>MSLSAKSSLKEVAELAGVGYATASRALSGKGYVSPQTREKVQAAAKELNYVPNQLAKALREHRSALVGVIVPDLSNEYYSESLQTIQQDLKAAGYQMLVAEANSVQAQDVVMESLISIQAAGIIHVPVVGSIAPEGIPMVQLTRGELGPGFPRVLCDDEAGFFQLTESVLGGSGMNIAALVGEESLSTTQERMRGISHAASIYGAEVTFHFGHYSVESGEEMAQVVFNNGLPDALIVASPRLMAGVMRAFTRLNVRVPHDVVIGGYDDPEWYSFVGAGITTFVPPHEEMGKEAVRLLVDLIENPELPTGDVVLQGQ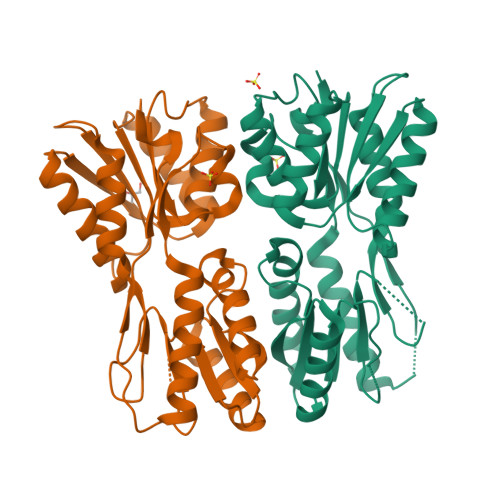VILRGSSTHEGHHHHHH[2x]>MENFPTEYFLNTTVRLLEYIRYRDSNYTREERIENLHYAYNKAAHHFAQPRQQQLLKVDPKRLQASLQTIVGMVVYSWAKVSKECMADLSIHYTYTLVLEDSKDDPYPTMVNYFDDLQAGREQAHPWWALVNEHFPNVLRHFGPFCSLNLIRSTLDFFEGCWIEQYNFGGFPGSHDYPQ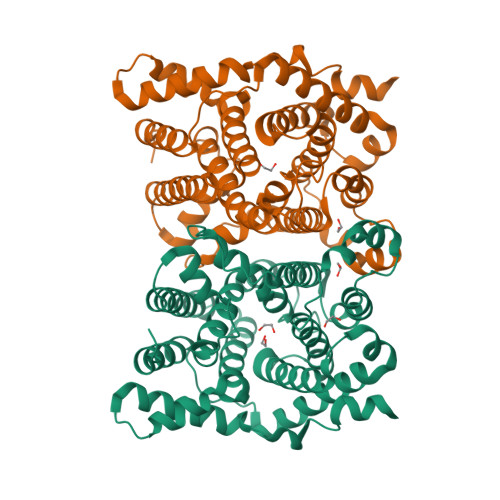FLRRMNGLGHCVGASLWPKEQFNERSLFLEITSAIAQMENWMVWVNDLMSFYKEFDDERDQISLVKNYVVSDEISLHEALEKLTQDTLHSSKQMVAVFSDKDPQVMDTIECFMHGYVTWHLCDRRYRLSEIYEKVKEEKTEDAQKFCKFYEQAANVGAVSPSEWAYPPVAQLANVRSKDVKEVQKPFLSSIELVE[2x]> MVENNALSLVARGCAVAAPCRTKVAEQLLEIGAKAGMAGLAGAAVKDMADRMTSDELEHLITLQMMGNDEITTKYLSSLHDKYGSGAASNPNIGKD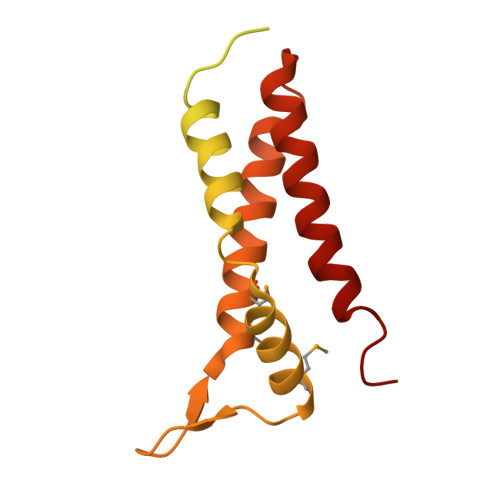LTDAEKVELGGSGSGTGTPPPSENDPKQQNEKTVDKLNQKQESAIKKIDNTIKNALKDHDIIGTLKDMDGKPVPKENGGYWDHMQEMQNTLRGLRNHADTLKNVNNPEAQAAYGRATDAINKIESALKGYGI>FQSMSVRPPVLVDIKFNPEGVDRVLKTAFADRGSINLADPANRERDFSETEYALLWKPDADLFRRAPNLKVIFSGGAGVDHIIGMAGLPDIPIVRFVDRSLTTRMSEWVVMQCLMHLRGQYGHDSHQRRREWAKLIAPEAAEVTVGVMGLGILGQDAVAKLKVMGFNVIGWSRTRKTIEGVETFDAGELDRFLAKTDILVGLLPLTPETTGFYDSELFKKLRRDGALGQPVFINAGRGKSQIETDIVSAVREGTLGGASLDVFEVEPLATDSPLWELENVFITPHDAAVSEENALFR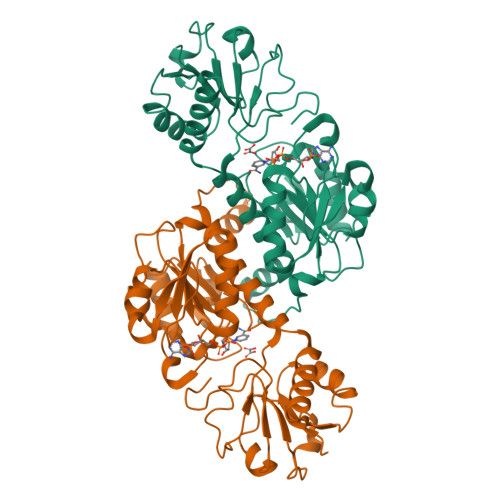HVEMQIARFERGEPLQFVIDRAAGY[2x]> MVEATAQETDRPRFSFSIAAREGKARTGTIEMKRGVIRTPAFMPVGTAATVMALKPETVRATGADIILGNTYHLMLRPGAERIAKLGGLHSFMGWDRPILTDSGGYQVMSLSSLTKQSEEGVTFKSHLDGSRHMLSPERSIEIQHLLGSDIVMAFDECTPYPATPSRAASSMERSMRWAKRSRDAFDSRKEQAENAALFGIQQGSVFENLRQQSADALAEIGFD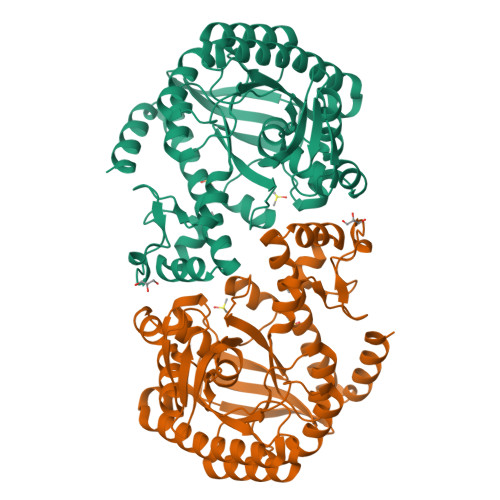GYAVGGLAVGEGQDEMFRVLDFSVPMLPDDKPHYLMGVGKPDDIVGAVERGIDMFDCVLPTRSGRNGQAFTWDGPINIRNARFSEDLKPLDSECHCAVCQKWSRAYIHHLIRAGEILGAMLMTEHNIAFYQQLMQKIRDSISEGRFSQFAQDFRARYFARNS>[2x]XLAACLC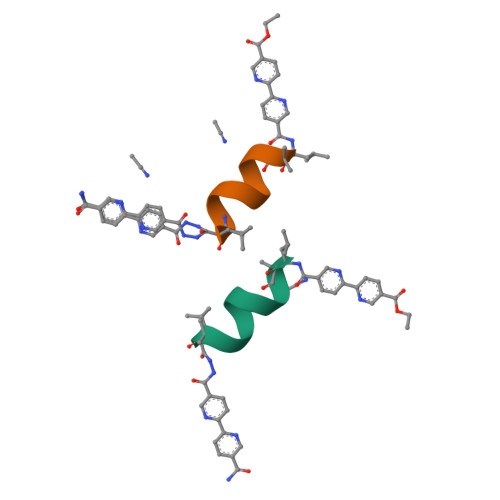QALX1,3-dihydroxypropan-2-yl 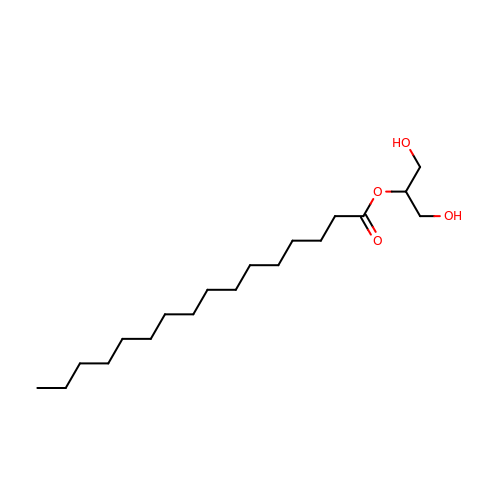hexadecanoate | C19 H38 O4 | BBNYCLAREVXOSG-UHFFFAOYSA-N> MLIEIHMIQNHSPANLNRDDLGAPKTCYFGGVLRSRISSQCIKRSIRTSNDFKALLGGVRTRRLADLIQQEAGETECWKKAQEILNKCGFKNKDDNTKMLVFMSKDKIKDLARIVLDNSLGLTEAAQQVANVIAQATLAPDIALCGRMLEPNDKDKDKKVKWSNTTVEAALQVAHAISTHIARP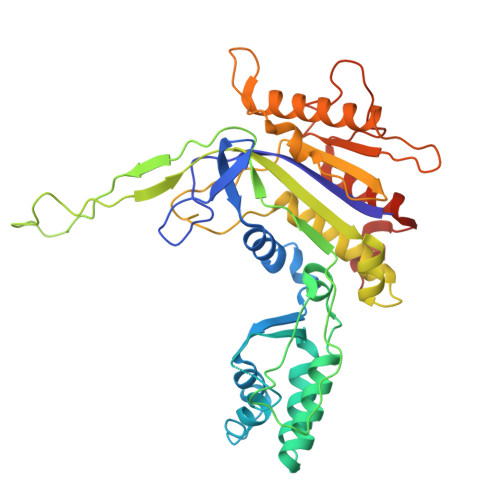EIDYFVAADDVPGEDAGAGHIGESMFASACFYKYFSIDWEQLVKNLKGDTNLAAHTVGAFLLAAAKTNPSGKQNSFAAHNYPDGILVEFKNSPISYANAFVRPVSVVKESDLVEQSIGQLSNYVNDIRLGYYDEQSPVIGFWFSPNNRYPLGYKHSKLASRNIGNLNELVGAVLDYIGGFKWEEVQKSKAYIGG> MARVT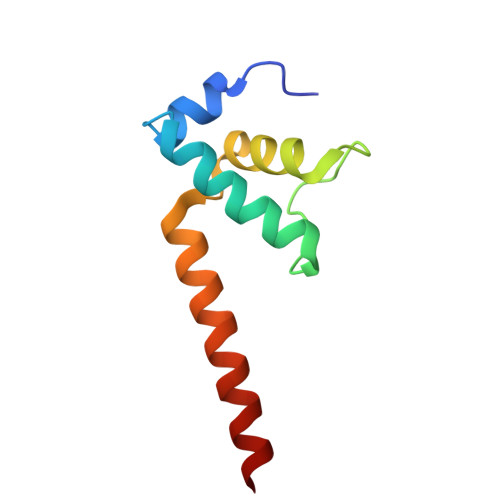VQDAVEKIGNRFDLVLVAARRARQMQVGGKDPLVPEENDKTTVIALREIEEGLINNQILDVRERQEQQEQEAAELQAVT> MGPHHHHHHLESTSLYKKAGSENLYFQSVAILQKRDHEGFGFVLRGAKAETPIEEFTPTPAFPALQYLES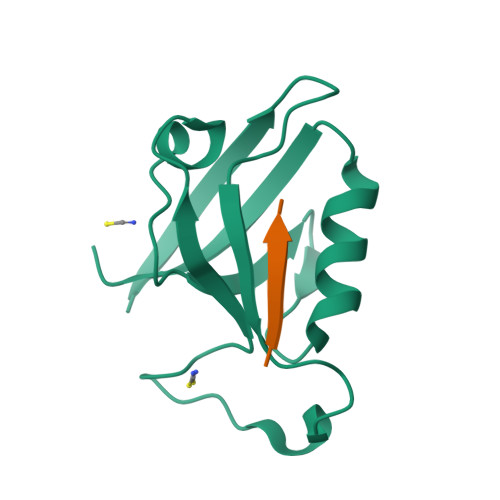VDVEGVAWKAGLRTGDFLIEVNGVNVVKVGHKQVVGLIRQGGNRLVMKVVSVT;> XIESTEI> MSLLNPVLLPPKVKAYLSQGERFIKWDDETTVASPVILRVDPKGYYLYWTYQSKEMEFLDITSIRDTRFGKFAKMPKSQKLRDVFNMDFPDNSFLLKTLTVVSGPDMVDLTFHNFVSYKENVGKAWAEDVLALVKHPLTANASRSTFLDKILVKLKMQLNSEGKIPVKNFFQMFPADRKRVEAALSACHLPKGKNDAINPEDFPEPVYKSFLMSLCPRPEIDEIFTSYHAKAKPYMTKEHLTKFINQKQRDSRLNSLLFPPARPDQVQGLIDKYEPSGINAQRGQLSPEGMVWFLCGPENSVLAQDKLLLHHDMTQPLNHYFINSSHNTYLTAGQFSGLSSAEMYRQVLLSGCRCVELDCWKGKPPDEEPIITHGFTMTTDIFFKEAIEAIAESAFKTSPYPIILSFENHVDSPRQQAKMAEYCRTIFGDMLLTEPLEKFPLKPGVPLPSPEDLRGKILIKNKKNQFSGPTSSSKDTGGEAEGSSPPSAPAVWAGEEGTELEEEEVEEEEEEESGNLDEEEIKKMQSDEGTAGLEVTAYEEMSSLVNYIQPTKFVSFEFSAQKNRSYVISSFTELKAYDLLSKASVQFVDYNKRQMSRIYPKGTRMDSSNYMPQMFWNAGCQMVALNFQTMDLPMQQNMAVFEFNGQSGYLLKHEFMRRPDKQFNPFSVDRIDVVVATTLSITVISGQFLSERSVRTYVEVELFGLPGDPKRRYRTKLSPSTNSINPVWKEEPFVFEKILMPELASLRVAVMEEGNKFLGHRIIPINALNSGYHHL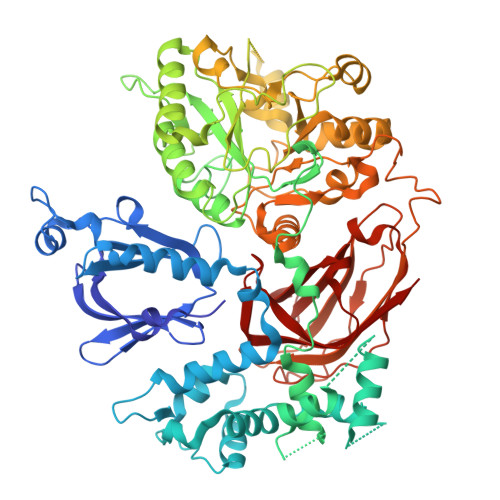CLHSESNMPLTMPALFIFLEMKD1-(2-carboxyphenyl)-7-chloro-6-[(2-chloro-4,6-difluorophenyl)amino]-4-oxo-1,4-dihydroquinoline-3-carboxylic 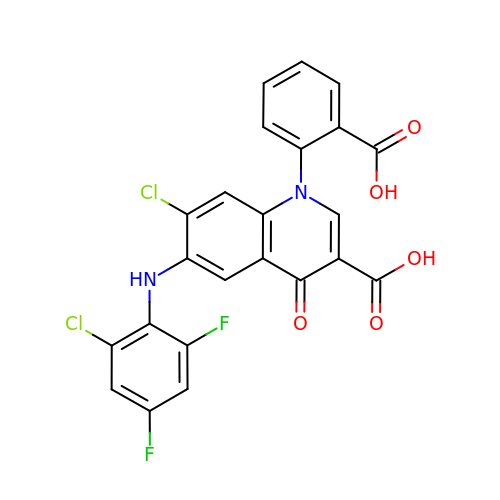acid | C23 H12 Cl2 F2 N2 O5 | OEMJXSVJXPIFMA-UHFFFAOYSA-N> MSLISKEELIKLAYSIRPRENEYKTILTNLDEYNKLTTNNNENKYLQLKKLNESIDVFMNKYKTSSRNRALSNLKKDILKEVILIKNSNTSPVEKNLHFVWIGGEVSDIALEYIKQWADINAEYNIKLWYDSEAFLVNTLKKAIVESSTTEALQLLEEEIQNPQFDNMKFYKKRMEFIYDRQKRFINYYKSQINKPTVPTIDDIIKSHLVSEYNRDETVLESYRTNSLRKINSNHGIDIRANSLFTEQELLNIYSQELLNRGNLAAASDIVRLLALKNFGGVYLDVDMLPGIHSDLFKTISRPSSIGLDRWEMIKLEAIMKYKKYINNYTSENFDKLDQQLKDNFKLIIESKSEKSEIFSKL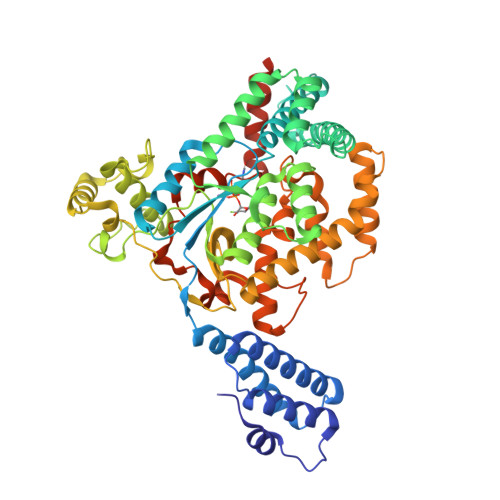ENLNVSDLEIKIAFALGSVINQALISKQGSYLTNLVIEQVKNRYQFLNQHLNPAIESDNNFTDTTKIFHDSLFNSATAENSMFLTKIAPYLQVGFMPEARSTISLSGPGAYASAYYDFINLQENTIEKTLKASDLIEFKFPENNLSQLTEQEINSLWSFDQASAKYQFEKYVRDYTGGSLSEPHAGLRGSHHHHHH> HHHHHHSSGLVPRGSKPFPAERIISLAPHATEIAYAAGLGDKLVAVS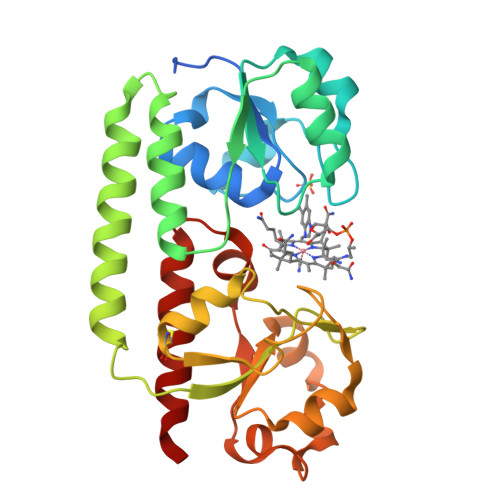EYSDYPPQALELERVANHQTINIEKILTLKPDLIIAWPAGNPPRELAKLRQLGFTIYDSQTKTLDEIADNIEALSHYSANPEVGQKAAHDFRQRLQDLRTQYASNQPIRYFYQLSEKPIITLAQGHWPSEVFSLCGGVNIFADSEVPYPQVSIEQVLVKQPQVIFTSEHAIANGHMWRAWQAELSAVQNDQVWALNADWLNRPTPRTLDAVEQVCTYLKIAQKQ>[2x]NVEEETKYIELMIVNDHLMFKKHRLSVVHTNTYAKSVVNMADLIYKDQLKTRIVLVAMETWATDNKFAISENPLITLREFMKYRRDFIKEKSDAVHLFSGSQFESSRSGAAYIGGICSLLKGGGVNEFGKTDLMAVTLAQSLAHNIGIISDKRKLASGECKCEDTWSGCIMGDTGYYLPKKFTQCNIEEYHDFLNSGGGACLFNKPSKLLDPPECGNGFIETGEECDCGTPAECVLEGAECCKKCTLTQDSQCSDGLCCKKCKFQPMGTVCREAVNDCDIRETCSGNSSQCAPNIHKMDGYSCDGVQGICFGGRCKTRDRQCKYIWGQKVTASDKYCYEKLNIEGTEKGNCGKDKDTWIQCNKRDVLCGYLLCTNIGNIPRLGELDGEITSTLVVQQGRTLNCSGGHVKLEEDVDLGYVEDGTPCGPQMMCLEHRCLPVASFNFSTCLSSKEGTICSGNGVCSNELKCVCNRHWIGSDCNTYFPHNDDAKTGITLSG;>DAAQPARRARRTYEAYPAKPKCPAVCTCTKDNALCENARSIPRTVPPDVISLSFVRSGFTEISEGSFLFTPSLQLLLFTSNSFDVISDDAFIGLPHLEYLFIENNNIKSISRHTFRGLKSLIHLSLANNNLQTLPKDIFKGLDSLTNVDLRGNSFNCDCKLKWLVEWLGHTNATVEDIYCEGPPEYKKRKINSLSSKDFDCIITEFAKSQDLPYQSLSIDTFSYLNDEYVVIAQPFTGKCIFLEWDHVEKTFRNYDNITGTSTVVCKPIVIETQLYVIVAQLFGGSHIYKRDSFANKFIKIQDIEILKIRKPNDIETFKIENNWYFVVADSSKAGFTTIYKWNGNGFYSHQSLHAWYRDTDVEYLEIVRTPQTLRTPHLILSSSSQRPVIYQWNKATQLFTNQTDIPNMEDVYAVKHFSVKGDVYICLTRFIGDSKVMKWGGSSFQDIQAMPSRGSMVFQPLQINNYQYAILGSDYSFTQVYNWDAEKAKFVKFQELNVQAPRSFTHVSINKRNFLFASSFKGNTQIYKHVIVDLSAKHHHHHH[2x]

LGI1 is a 60-kDa secreted neuronal protein, which consists of the N-terminal leucine-rich repeat (LRR) domain and the C-terminal epitempin-repeat (EPTP) (also known as EAR) domain4. ADAM22 serves as a receptor for LGI1 and is anchored to the excitatory postsynaptic density through PSD-95 scaffold. The LGI1–ADAM22 ligand–receptor interaction plays an essential role in AMPA-type glutamate receptor-mediated synaptic transmission via PSD-9533–35. In this study, we present the crystal structures of LGI1 LRR, LGI1 EPTP–ADAM22, and LGI1–ADAM22 at 1.78, 2.67, and 7.13 Å resolutions, respectively.

We coincidentally found that the R470A mutation of LGI1 enhances the expression level of the complex. The crystal structure of the LGI1R470A–ADAM22 ECD complex was determined at 7.13 Å resolution by molecular replacement using the crystal structures of the LGI1 EPTP–ADAM22 ECD complex and LGI1 LRR as the search models. The LGI1–ADAM22 complex structure forms a 2:2 heterotetramer in the asymmetric unit of the crystal. The length along the longest axis of the 2:2 LGI1–ADAM22 complex is about 190 Å, which is equivalent to the length of a synaptic cleft. Two copies of the 1:1 LGI1–ADAM22 complex are aligned in a head-to-head configuration with ~90° rotation along the longest axis. The LRR and EPTP domains of LGI1 are connected by a 2-residue linker (Ile222–Ile223) and adopt an extended conformation. LGI1 EPTP interacts with the metalloprotease-like domain of ADAM22 in the same manner as in the LGI1 EPTP–ADAM22 ECD complex, whereas the LRR domain of one LGI1 molecule interacts with the EPTP domain of the other LGI1 molecule, thereby bridging two distant ADAM22 molecules in the complex. The C-terminals of the two ADAM22 molecules are oriented in the opposite directions. The high-resolution structures of the LGI1 EPTP–ADAM22 ECD complex and LGI1 LRR allowed us to interpret the 7.13-Å-resolution map and obtain the information of the intermolecular interactions between LRR and EPTP and that between LRR and ADAM22 ECD in the 2:2 heterotetrameric LGI1–ADAM22 complex: Glu123 and Arg76 in the LRR domain of one LGI1 likely form hydrogen bonds with Arg474 and Glu516 in the EPTP domain of the other LGI1, respectively. His116 of LGI1 LRR likely interacts with Glu446 in the disintegrin domain of ADAM22. It should be noted that two human ADLTE mutations, E123K17 and aforementioned R474Q, occur in the interface of the LGI1–LGI1 interaction in the 2:2 LGI1–ADAM22 complex.> ADVPAGVQLADKQTLVRNNGSEVQSLDPHKIEGVPESNVSRDLFEGLLISDVEGHPSPGVAEKWENKDFKVWTFHLRENAKWSDGTPVTAHDFVYSWQRLADPNTASPYASYLQYGHIANIDDIIAGKKPATDLGVKALDDHTFEVTLSEPVPYFYKLLVHPSVSPVPKSAVEKFGDKWTQPANIVTNGAYKLKNWVVNERIVLERNPQYWDNAKTVINQVTYLPISSEVTDVNRYRSGEIDMTYNNMPIELFQKLKKEIPNEVRVDPYLCTYYYEINNQKAPFNDVRVRTALKLALDRDIIVNKVKNQGDLPAYSYTPPYTDGAKLVEPEWFKWSQQKRNEEAKKLLAEAGFTADKPLTFDLL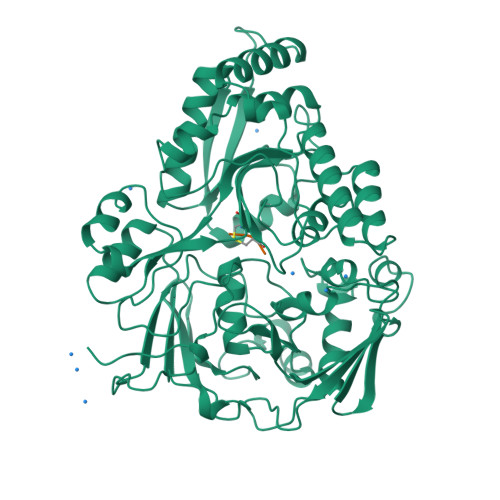YNTSDLHKKLAIAVASIWKKNLGVNVNLENQEWKTFLDTRHQGTFDVARAGWCADYNEPTSFLNTMLSDSSNNTAHYKSPAFDKLIADTLKVADDTQRSELYAKAEQQLDKDSAIVPVYYYVNARLVKPWVGGYTGKDPLDNIYVKNLYIIKH;> KHK> MSEMSYLEKLLDGVEVEWLPLGEITKYEQPTKYLVKAKDYHDTYTIPVLTAGKTFILGYTNETHGIYQASKAPVIIFDDFTTANKWVDFDFKAKSSAMKMVTSCDDNKTLLKYVYYWLNTLPSEFAEGDHKRQWISNYSQKKIPI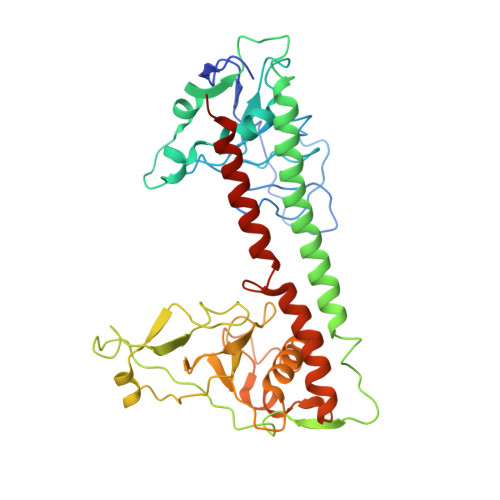PCPDNPEKSLAIQSEIVRILDKFTALTAELTAELNMRKKQYNYYRDQLLSFKEGEVEWKTLGEIGKWYGGGTPSKNKIEFWENGSIPWISPKDMGRTLVDSSEDYITEEAVLHSSTKLIPANSIAIVVRSSILDKVLPSALIKVPATLNQDMKAVIPHENILVKYIYHMIGSRGSDILRAAKKTGGSVASIDSKKLFSFKIPVPNINEQQRIVEILDKFDTLTNSITEGLPREIELRQKQYEYYRDLLFSFPKPETVSN> MTHDNKLQVEAIKRGTVIDHIPAQIGFKLLSLFKLTETDQRITIGLNLPSGEMGRKDLIKIENTFLSEDQVDQLALYAPQAAVNRIDNYEVVGKSRPSLPERIDNVLVCPNSNCISHAEPVSSSFAVRKRANDIALKCKYCEKEF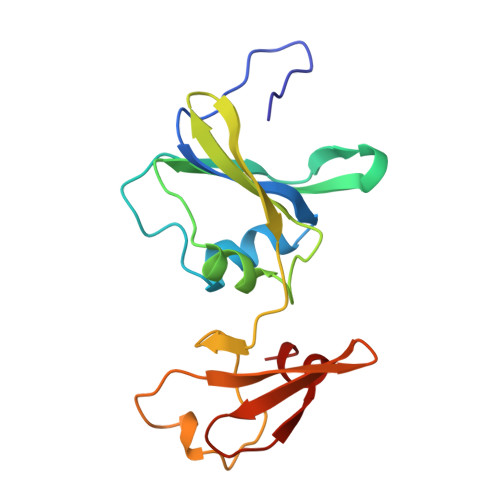SHNVVLAN> MYINNGRINYNNEYGYRRGIYREPFYSDNADYNTNSKSYYDYLARFNGFIFELCDFVNGLADDIQKMKDTYEALTLSNTDVTYTVGQKGDFDTLNHCFEHIEDLIVQPKSIRVILLKDYMMREQLFLRDKRYNHITITSENDIVEAYETELNRQVEIKTNPIFRVKPLFYGINSTFPKIDFKLQNKDFSDTINCGFLMDNTTFE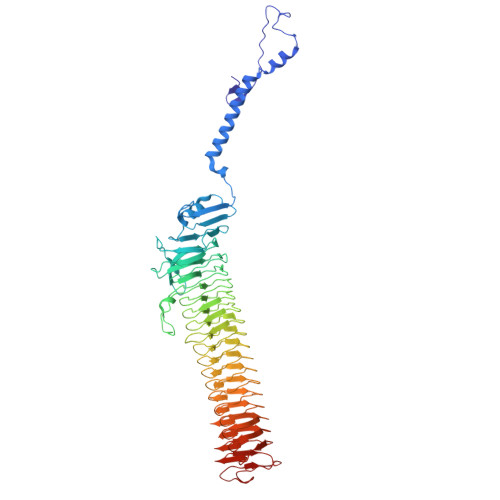MTERGGSTHFNFIGLCGVNGSHIQTNYCDFSYNGNREQLEEYNKDQNMYGDGLRIFNSSLTGNYMTVNRCGEIGIHFSHGASGYIDFTEARFNGHHGLMVTTGSQASARNCKITDTIDDNVVSYASSDIDLRSSDCSNSQTTYGVIATRSSNINFDKGIANGCGASGIMANRGCSIDATGATASRNKWHGVIASNNSKVDFTSGNANENGLDGIQCTHGSTVQARLSTTNGNKRNGVLAYAGDVYCQEINCDGNGRRGLEATRGGYVAAYGAKVSRSKDDNVLAYGSMISINEALIERAGRNGIEATRGGQIFADRITITGSGDFGILAYASKVFAEASNISGTKNEPVYATRGGEVTCFGSNISSNKTVYNVYNGSRIFTDKDHGYSTNVDPQTLSSKGLIILG> APSASFERRQGSVNPYIGRSPLVIKSYAEKLEETIAYFEAQGDELNAARTRTVQGIPTFAWISDSATIDTIQPLIADAVAHQEASGEQVLVQLVIYNLPDRACAAKASDGEFHLDDDGANKYRAYVDRIVAELSTADADKLHFSIVLEPDSLGNMVTNMHVPKCQGAATAYKEGIAYTIASLQKPNIDLYIDAAHG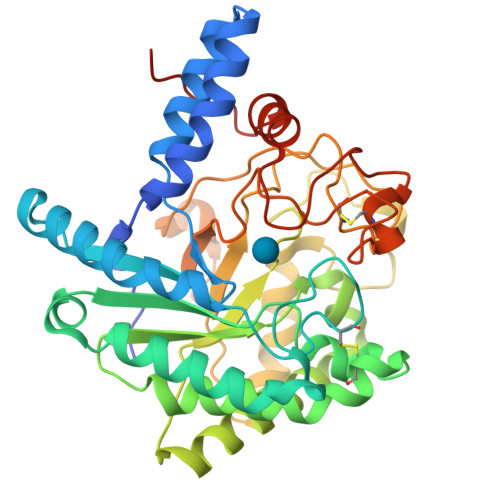GWLGWNDNLRPSAEIFKETLDLARQITPNATVRGLAINVSNYNPYKTRAREDYTEWNNAYDEWNYVKTLTPHLQAVGFPAQFIVDQGRSGREGIRTEWGQWCNIRNAGFGIRPTTDQAIVDSANVDAIVWVKPGGESDGTSDVNAVRFDENCRSPASHVPAPEAGEWFNEFVVNLVINANPPLEPTYAAAALEHHHHHH Parasite-infected red blood cells sequester in the placenta through interaction between parasite-expressed protein VAR2CSA and the glycosaminoglycan chondroitin sulfate A (CS) abundantly present in the intervillous space. Here, we report cryo-EM structures of the VAR2CSA ectodomain at up to 3.1 Å resolution revealing an overall V-shaped architecture and a complex domain organization. Compared to other PfEMP1s, the ~310 kDa VAR2CSA ectodomain is relatively conserved among parasites. It is composed of a short N-terminal segment and six Duffy Binding-Like (DBL) domains (DBL1-DBL6) unique to VAR2CSA. Several of the DBL domains are linked by complex inter-domain (ID1-3) regions with limited or no homology among PfEMP1s yielding a DBL1-ID1-DBL2-ID2-DBL3-DBL4-ID3-DBL5-ID4-DBL6 structure.

Likewise, the C-terminal DBL5 and DBL6 are more separated from the core, linking the protein to the membrane in a physiological setting. The DBL5 and DBL6 form a rod-like structure with weak inter-domain contacts. Flexibility of these domains is further supported by two separately generated maps based on different subsets of particles, showing the same core structure, but different conformations of DBL5/DBL6. By contrast, DBL1 and DBL5/6 were less well resolved compared to the apo structure. The simulations also suggested significant flexibility of DBL1 and DBL5/6, consistent with the relatively poor EM density in these regions.

> MDSTSTIANKIEEYLGAKSDDSKIDELLKADPSEVEYYRSGGDGDYLKNNICKITVNHSDSGKYDPCEKKLPPYDDNDQWKCQQNSSDGSGKPENICVPPRRERLCTYNLENLKFDKIRDNNAFLADVLLTARNEGEKIVQNHPDTNSSNVCNALERSFADLADIIRGTDQWKGTNSNLEKNLKQMFAKIRENDKVLQDKYPKDQKYTKLREAWWNANRQKVWEVITCGARSNDLLIKRGWRTSGKSDRKKNFELCRKCGHYEKEVPTKLDYVPQFLRWLTEWIEDFYREKQNLIDDMERHREECTREDHKSKEGTSYCSTCKDKCKKYCECVKKWKTEWENQENKYKDLYEQNKNKTSQKNTSRYDDYVKDFFEKLEANYSSLENYIKGDPYFAEYATKLSFILNPSDANNPSGETANHNDEACNCNESGISSVGQAQTSGPSSNKTCITHSSIKTNKKKECKDVKLGVRENDKDLKICVIEDTSLSGVDNCCCQDLLGILQENCSDNKRGSSSNDSCDNKNQDECQKKLEKVFASLTNGYKCDKCKSGTSRSKKKWIWKKSSGNEEGLQEEYANTIGLPPRTQSLYLGNLPKLENVCEDVKDINFDTKEKFLAGCLIVSFHEGKNLKKRYPQNKNSGNKENLCKALEYSFADYGDLIKGTSIWDNEYTKDLELNLQNNFGKLFGKYIKKNNTAEQDTSYSSLDELRESWWNTNKKYIWTAMKHGAEMNITTCNADGSVTGSGSSCDDIPTIDLIPQYLRFLQEWVENFCEQRQAKVKDVITNCKSCKESGNKCKTECKTKCKDECEKYKKFIEACGTAGGGIGTAGSPWSKRWDQIYKRYSKHIEDAKRNRKAGTKNCGTSSTTNAAASTDENKCVQSDIDSFFKHLIDIGLTTPSSYLSNVLDDNICGADKAPWTTYTTYTTTEKCNKERDKSKSQSSDTLVVVNVPSPLGNTPYRYKYACQCKIPTNEETCDDRKEYMNQWSCGSARTMKRGYKNDNYELCKYNGVDVKPTTVRSNSSKLDGNDVTFFNLFEQWNKEIQYQIEQYMTNANISCIDEKEVLDSVSDEGTPKVRGGYEDGRNNNTDQGTNCKEKCKCYKLWIEKINDQWGKQKDNYNKFRSKQIYDANKGSQNKKVVSLSNFLFFSCWEEYIQKYFNGDWSKIKNIGSDTFEFLIKKCGNNSAHGEEIFSEKLKNAEKKCKENESTDTNINKSETSCDLNATNYIRGCQSKTYDGKIFPGKGGEKQWICKDTIIHGDTNGACIPPRTQNLCVGELWDKSYGGRSNIKNDTKELLKEKIKNAIHKETELLYEYHDTGTAIISKNDKKGQKGKNDPNGLPKGFCHAVQRSFIDYKNMILGTSVNIYEHIGKLQEDIKKIIEKGTPQQKDKIGGVGSSTENVNAWWKGIEREMWDAVRCAITKINKKNNNSIFNGDECGVSPPTGNDEDQSVSWFKEWGEQFCIERLRYEQNIREACTINGKNEKKCINSKSGQGDKIQGACKRKCEKYKKYISEKKQEWDKQKTKYENKYVGKSASDLLKENYPECISANFDFIFNDNIEYKTYYPYGDYSSICSCEQVKYYKYNNAEKKNNKSLCYEKDNDMTWSKKYIKKLENGRSLEGVYVPPRRQQLCLYELFPIIIKNEEGMEKAKEELLETLQIVAEREAYYLWKQYNPTGKGIDDANKKACCAIRGSFYDLEDIIKGNDLVHDEYTKYIDSKLNEIFGSSNTNDIDTKRARTDWWENETITNGTDRKTIRQLVWDAMQSGVRYAVEEKNENFPLCMGVEHIGIAKPQFIRWLEEWTNEFCEKYTKYFEDMKSKCDPPKRADTCGDNSNIECKKACANYTNWLNPKRIEWNGMSNYYNKIYRKSNKESEDGKDYSMIMAPTVIDYLNKRCHGEINGNYICCSCKNIGAYNTTSGTVNKKLQKKETECEEEKGPLDLMNEVLNKMDKKYSAHKMKCTEVYLEHVEEQLNEIDNAIKDYKLYPLDRCFDDQTKMKVCDLIADAIGCKDKTKLDELDEWNDMDLRGTYNKHKGVLIPPRRRQLCFSRIVRGPANLRSLNEFKEEILKGAQSEGKFLGNYYKEHKDKEKALEAMKNSFYDYEDIIKGTDMLTNIEFKDIKIKLDRLLEKETNNTKKAEDWWKTNKKSIWNAMLCGYKKSGNKIIDPSWCTIPTTETPPQFLRWIKEWGTNVCIQKQEHKEYVKSKCSNVTNLGAQASESNNCTSEIKKYQEWSRKRSIQWETISKRYKKYKRMDILKDVKEPDANTYLREHCSKCPCGFNDMEEMNNNEDNEKEAFKQIKEQVKIPAELEDVIYRIKHHEYDKGNDYICNKYKNIHDRMKKNNGNFVTDNFVKKSWEISNGVLIPPRRKNLFLYIDPSKICEYKKDPKLFKDFIYWSAFTEVERLKKAYGGARAKVVHAMKYSFTDIGSIIKGDDMMEKNSSDKIGKILGDTDGQNEKRKKWWDMNKYHIWESMLCGYREAEGDTETNENCRFPDIESVPQFLRWFQEWSENFCDRRQKLYDKLNSECISAECTNGSVDNSKCTHACVNYKNYILTKKTEYEIQTNKYDNEFKNKNSNDKDAPDYLKEKCNDNKCECLNKHIDDKNKTWKNPYETLEDTFKSKCDCPKPLPSPIKPDDLPPQADEPF> RPIRLLPWLQVVKIGGRVMDRGADAILPLVEELRKLLPEHRLLILTGAGVRARHVFSVGLDLGLPVGSLAPLAASEAGQNGHILA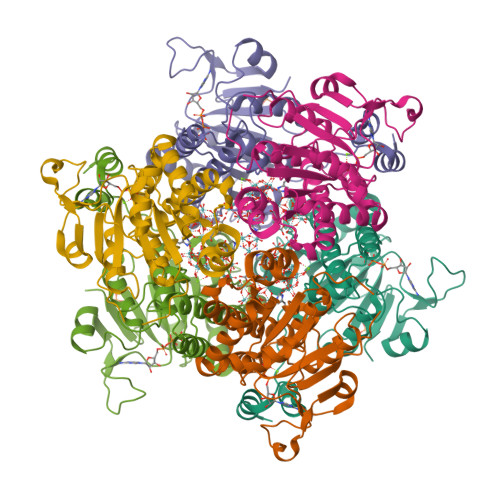AMLASEGVSYVEHPTVADQLAIHLSATRAVVGSAFPPYHHHEFPGSRIPPHRADTGAFLLADAFGAAGLTIVENVDGIYTADPNGPDRGQARFLPETSATDLAKSEGPLPVDRALLDVMATARHIERVQVVNGLVPGRLTAALRGEHVGTLIRTGVRPA;> NSTAELEELLMQRSLTDPQLQAAAAAAADFRILPDATVIKIGGQSVIDRGRAAVYPLVDEIVAARKNHKLLIGTGAGTRARHLYSIAAGLGLPAGVLAQLGSSVADQNAAMLGQLLAKHGIPVVGGAGLSAVPLSLAEVNAVVFSGMPPYKLWMRPAAEGVIPPYRTDAGCFLLAEQFGCKQMIFVKDEDGLYTANPKTSKDATFIPRISVDEMKAKGLHDSILEFPVLDLLQSAQHVREVQVVNGLVPGNLTRALAGEHVGTIITAS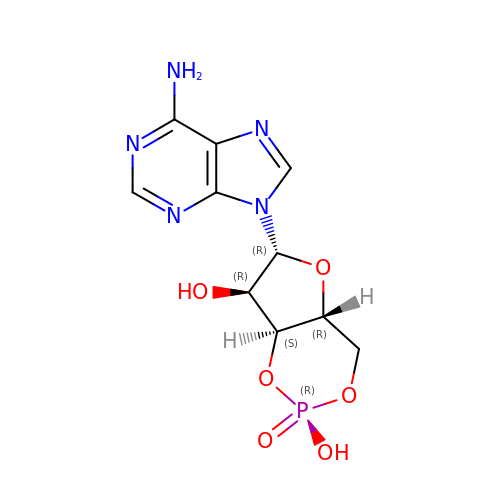ADENOSINE-3',5'-CYCLIC-MONOPHOSPHATE | C10 H12 N5 O6 P | IVOMOUWHDPKRLL-KQYNXXCUSA-N1-{4-[5-({3-[(2-methylpyridin-3-yl)oxy]-5-[(pyridin-2-yl)sulfanyl]pyridin-2-yl}amino)-1,2,4-thiadiazol-3-yl]piperidin-1-yl}ethan-1-one 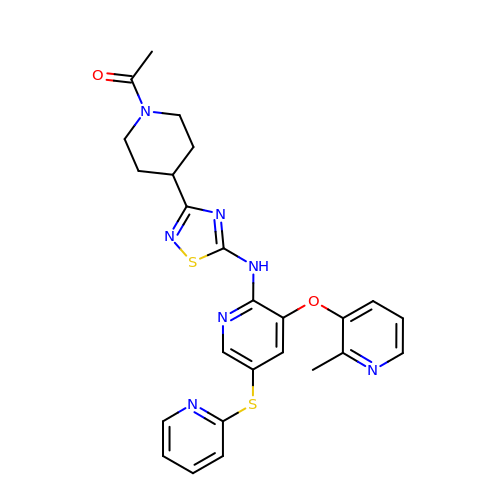| C25 H25 N7 O2 S2 | WITGITFYEMHCEZ-UHFFFAOYSA-N> YVEFAQDFDFFYFVQQWPASYCDTRRSCCYPTTGKPDEDFSIHGLWPNYENGKWPQNCDRESSLDESEISDLISTMEKNWPSLACPSSDGVRFWSHEWLKHGTCSALGERAYFQAALDFRKKSNLLENLKNAEITPRNGEHYTLESIKKAIEEGVGHSPYIECNVDTQGNHQIYQVYLCVD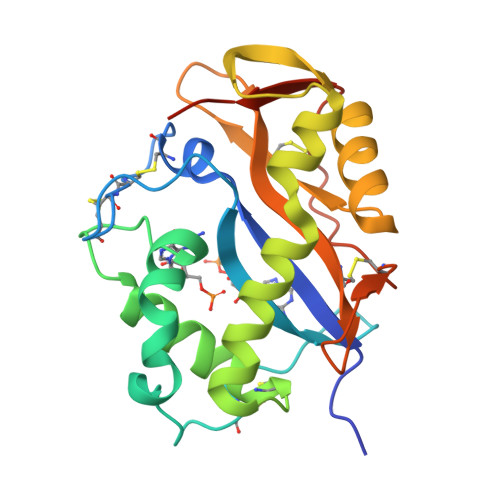KTATDFIDCPIFPHGRGCGSKIEFPPFSSESDHDEF> PDCGVECKNETCTPKTVIYPDCGKNEKYEPPGDAKNTEINVINSGDKEGYIFEKLSEFCTNENNENGKNYEQWKCYYDNKKNNNKCKMEINIANSKLKNK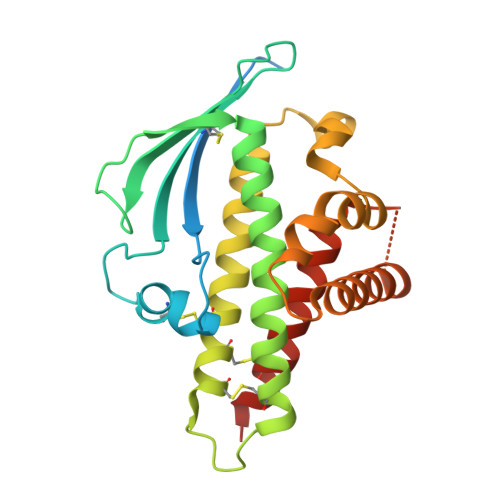VTSFDEFFDFWVRKLLIDTIKWETELTYCINNTDVTDCNKCNKNCVCFDKWVKQKEDEWTNIMKLFTNKHDIPKKYYLNINDLFDSFFFQVIYKFNEGEAKWNELKENLKKQIASSKANNGTKDSEAAIKVLFNHIKEIATICKDNNTNEG> EDIKVAVVGAMSGPVAQYGDQEFTGAEQAVADINAKGGIKGNKLQ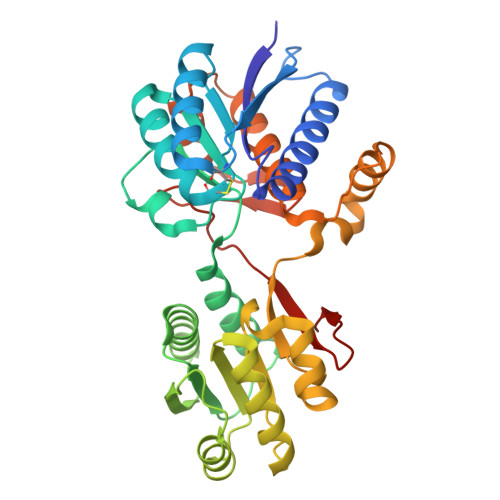IVKYDDACDPKQAVAVANKVVNDGIKYVIGHLCSSSTQPASDIYEDEGILMITPAATAPELTARGYQLILRTTGLDSDQGPTAAKYILEKVKPQRIAIVHDKQQYGEGLARAVQDGLKKGNANVVFFDGITAGEKDFSTLVARLKKENIDFVYYGGYHPEMGQILRQARAAGLKTQFMGPEGVANVSLSNIAGESAEGLLVTKPKNYDQVPANKPIVDAIKAKKQDPSGAFVWTTYAALQSLQAGLNQSDDPAEIAKYLKANSVDTVMGPLTWDEKGDLKGFEFGVFDWHANGTATDAK> GGYVAPKAVWLPAVKAKGLEISGTFTHRQGHIYMEMNFTNKALQHMTDFAIQ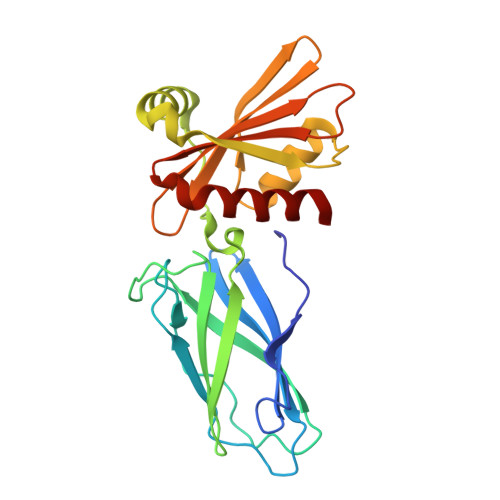FNKNSFGVIPSTPLAIHTPLMPNQSIDVSLPLNTLGPVMKMEPLNNLQVAVKNNIDVFYFSCLIPLNVLFVEDGKMERQVFLATWKDIPNENELQFQIKECHLNADTVSSKLQNNNVYTIAKRNVEGQDMLYQSLKLTNGIWILAELRIQPGNPNYTLSLKCRAPEVSQYIYQVYDSILKN> MATNFFIQPITEEAEAYYPPSVITNKRKDLGVDVYCCSDLVLQPGLNIVRLHIKVACEHMGKKCGFKIMARSSMCTHERLLILANGIGLIDPGYVGELMLKIINLGDTPVQIWAKECLVQLVAQGDHVPDHINILKRNQIFPLFAPTPRGEGRFGSTGEAGIMRT

Deoxyuridine 5'-triphosphate nucleotidohydrolase (dUTPase, EC 3.6.1.23) is a ubiquitous enzyme in DNA repair that plays a key role in preventing uracil from being incorporated into DNA. dUTPases are widespread in organisms, including eukaryotes, prokaryotes, and some viruses. On the one hand, it catalyzes the cleavage of dUTP into dUMP and pyrophosphate (PPi), which reduces the possibility that dUTP will be incorporated into DNA through DNA polymerase. Herein, we determine the crystal structures of ASFV dUTPase and swine dUTPase in both their ligand-free and ligand-bound forms. We observe that the swine enzyme employs a classical dUTPase architecture made up of three-subunit active sites, whereas the ASFV enzyme employs a novel two-subunit active site.

ASFV dUTPase (aDUT) gene consists of 495 bp and encodes 165 amino acid residues. The results of gel filtration experiments on the recombinant protein and static light scattering measurements indicated that ASFV dUTPase is in a trimeric conformation, which is consistent with the results of previous studies. Ligand-free ASFV dUTPase crystals grew in the I213 space group with a subunit in each asymmetric unit, and the structure contained 146 visible residues (residues 1–146); the remaining C-terminal residues (residues 147–165) are flexible. Comparison of the prereaction state and quiescent state showed a root-mean-square deviation (RMSD) of 0.519 Å for the active sites. These differences are evidence of the conformational changes induced by dUTP binding, as active-site residues are rearranged to provide a tight pocket for the substrate. Comparison of the postreaction state and quiescent state showed an RMSD of 0.364 Å for the active sites, suggesting that the conformational changes are also beneficial to the release of the product. The results of the thermofluor assay showed that ASFV dUTPase was denatured when heated to approximately 83 °C, whereas swine dUTPase denatured at 62 °C, indicating that ASFV dUTPase had better thermal stability.> MAKRPTETERCIESLIAIFQKHAGRDGNNTKISKTEFLIFMNTELAAFTQNQKDPGVLDRMMKKLDLDSDGQLDF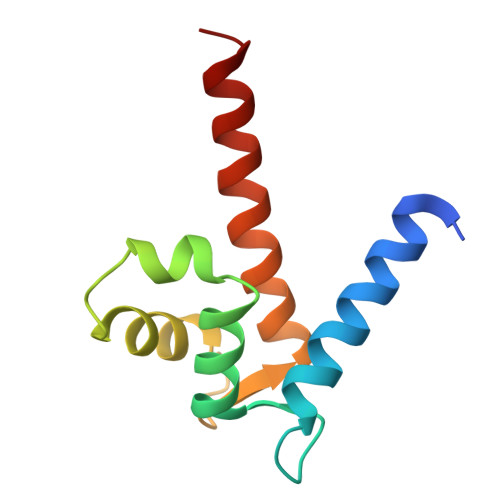QEFLNLIGGLAIACHDSFIKSTQK> SNAMFLKKKLSAGKSVVGTMLNLVYNPDIVR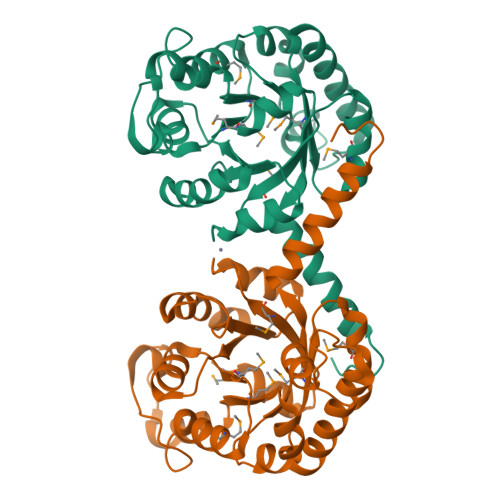IYAEAGLDYFIVDCEHAAYTFREINHLVSVAKNAGVSVLVRIPQVDRAHVQRLLDIGAEGFMIPGVQSAETMRETVRLAKYPPLGERGVGGSIVTDFKPVNWAEWVQERNDEIFIMAQIEHVKAVEDIDSILAVQGVDAVIFGPRDLSNDLGIIGQTEHPKVYECYEKVYRAADRQGVVKGFFTAADAAKMGWAVERGAQMLLWSGDVAALQTYTAKGVKTIKELPGFNP Botulinum neurotoxins (BoNTs), the most poisonous biological toxins for mammals, are speculated to exploit a similar mechanism to block neurotransmitter release at neuromuscular junctions that results in fatal botulism. A BoNT molecule consists of a light chain (LC) and a heavy chain (HC) that are linked by a disulfide bridge. LC is a zinc-dependent endopeptidase that is delivered into the cytosol where it degrades SNARE proteins to inhibit synaptic vesicle exocytosis. Membrane translocation of LC is mediated by HC, which can be subdivided into a translocation domain (HN) and a receptor-binding domain (HC).

Interestingly, diffraction-quality crystals of tHNA could only be obtained at an acidic pH despite thorough crystallization screens at various pH. We suspected that the isolated tHNA domain may be prone to adopting the acidic pH conformation needed for LC translocation, and its neutral pH conformation could be stabilized by LC/A and/or HCA. Taking advantage of our new crystal structure, we set out to look for point mutations on tHNA that shift the structural equilibrium of tHNA more towards the neutral pH conformation as opposed to the acidic pH conformation. After extensive search and screening, we found that tHNA carrying a single point mutation of F658E could be crystallized at pH 8.5 and we determined its structure at 3.02 Å. This result is consistent with our structural analysis that suggested F658E may destabilize the acidic pH conformation, but does not directly affect the neutral pH conformation. We found that the structure of tHNAF658E is highly similar to the corresponding region in full-length BoNT/A that was crystallized at a neutral pH (root-mean-square deviation of ~0.96 Å). Notably, the BoNT-switch adopts an almost identical structure in tHNAF658E and the full-length toxin. Taken together, the structures of tHNA at pH 5.1 and tHNAF658E at pH 8.5 allow us to directly visualize how the environmental pH regulates the conformation of the BoNT-switch. BoNT/A1F658E has a ~5-fold decreased toxicity, which is likely due to the energetic costs of burying of an acidic residue in a hydrophobic pocket when tHNA transits into the acidic-pH conformation during LC translocation.

> GPKYTMFHYLRAQEFEHGKSRIALTNSVNEALLNPSRVYTFFSSDYVKKVNKATEAAMFLGWVEQLVYDFTDETSEVSTTDKIADITIIIPYIGPALNIGNMLYKDDFVGALIESGAVILLEFIPEIAIPVLGTFALVSYIANKVLTVQTIDNALSKRNEKWDEVYKYIVTNWLAKVNTQIDLIRKKMKEALENQAEATKAIINYQYNQYTEEEKNNINFNIDDLSSKLNESINKAMININKFLNQCSVSYLMNSMIPYGVKRLEDFDASLKDALLKYIYDNRGTLIGQVDRLKDKVNNTLSTDIPFQLSKYVDNQRLLSTFTEYIK>[6x]GSMSTTDSRSATKSSSISPRHGRVITPESRAVYLYEAGRLDFGQVNELEGGKFFPATQSGLRDPDAPDDVANGMPPRD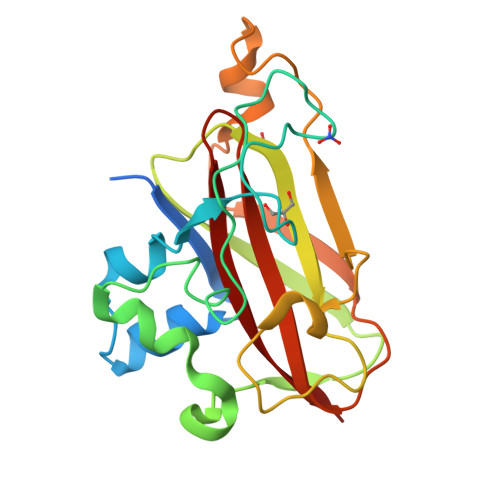GEIASGGRTADARAQLNEPDSVAHWQKHAVRSGQSLQISWSYSMPHKTRRWTYWITKPGWDTQARLARAHFEPDPLKVYLNTYQPYWGPDADKELIPQGETIHEFNLPTRTGYHVLLAVWDVADTANAFYQVIDLNFA>[2x]MII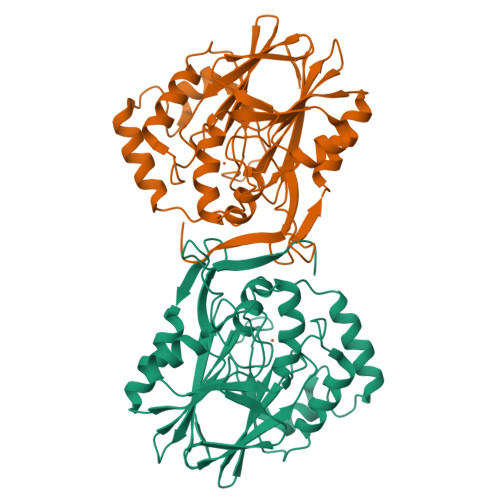GNNLHVDAFYDEATSTISYLVMDRETRQCALIDSVLDYDPKSGRTCSASADRLVERVNELNASVRWVLETHVHADHLSAAAYLKEKLGGHTAIGAHITQVQKVFGALFNAEPGFARDGSQFDVLLEDEEGFRIGNLQARALHTPGHTPACMSFMIEDAGEIAVFVGDTLFMPDYGTARCDFPGADARTLYRSIRRLLAFPDQTRLFMCHDYLPGGRDMQYVTTVAEQRASNIHIHQGIDEDSFVAMREARDKTLEMPVLILPSVQVNMRSGQLPPPEANGVSYLKIPLNKL>[2x]MQYDDDWQYEDCKLARDGPPATIVAIDEESRNGTILVDNMLIKGTAGGPDPTIELSLKDNVDYWVLMDPVKQMLFLNSTGRVLDRDPPMNIHSIVVQVQCINKKVGTIIYHEVRIVVRDRNDNSPTFKHESYYATVNELTPVGTTIFTGFSGDNGATDIDDGPNGQIEYVIQYNPDDPTSNDTFEIPLMLTGNIVLRKRLNYEDKTRYFVIIQANDRAQNLNERRTTTTTLTVDVLDGDDLGPMFLPCVLVPNTRDCRPLTYQAAIPELRTPEELNPIIVTPPIQAIDQDRNIQPPSDRPGILYSILVGTPEDYPRFFHMHPRTAELSLLEPVNRDFHQKFDLVIKAEQDNGHPLPAFAGLHIEILDENDNLEHHHHHH;>[2x]MQVNRLPFFTNHFFDEYLLISEDTPVGSS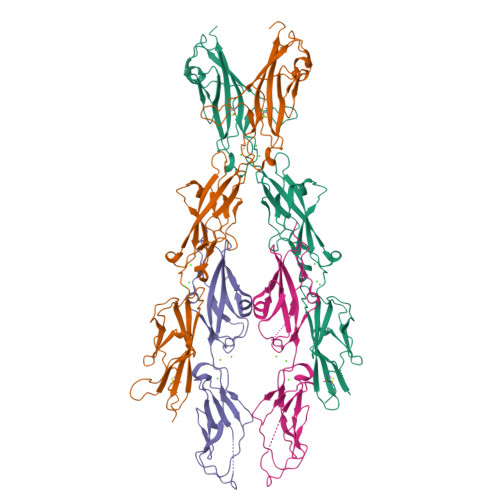VTQLLARDMDNDPLVFGVSGEEASRFFAVEPDTGVVWLRQPLDRETKSEFTVEFSVSDHQGVITRKVNIQVGDVNDNAPTFHNQPYSVRIPENTPVGTPIFIVNATDPDLGAGGSVLYSFQPPSPFFAIDSARGIVTVIQELDYEVTQAYQLTVNATDQDKTRPLSTLANLAIIITDLEHHHHHH>[4x]MGMSEPCHATIAELQAGIASGAYSREDVVAAHLGRTERINPVTNSYCELRGDQVLAEARAADREYGRELSGPLDGVPMSIKDSFAVRGLRRTDGLPVHADRVADEDDEVVARLRDAGGLVLGHANVPDICIRWNTISGLYGI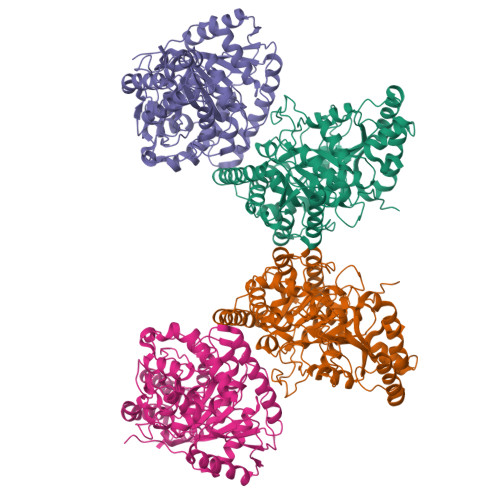ARNPRDPSRTAGGSSGGDAANVAAGMATVGMGQDLGGSIRVPASFCGVYGLRPGAGTVPNLSVIPPFPASPTLDAMGTSGPFARSAADLRTMFSVIAGAHPHDPVSVPAPLAGTASPRVAVLRGETGAVLDAEIEARLDATVDALRRAGFEVAEDVVPDLRRAPEVWAAINGTELINIALPEVGAEMTGSGRQHIEDMFGIFDLGLDLRAYHAVWLERRALQDALVRFLEDYPIIVAPVAGMPAPPLDFDHLIGREASARLFDRMRCVPWVNLFGLPGLALPNGIQLVTRRFHEPDLLATAEAIEPLLPAVEVADPVLEHHHHHH The PfEMP1 family of surface proteins is central for Plasmodium falciparum virulence and must retain the ability to bind to host receptors while also diversifying to aid immune evasion. The interaction between CIDRα1 domains of PfEMP1 and endothelial protein C receptor (EPCR) is associated with severe childhood malaria. We combine crystal structures of CIDRα1:EPCR complexes with analysis of 885 CIDRα1 sequences, showing that the EPCR-binding surfaces of CIDRα1 domains are conserved in shape and bonding potential, despite dramatic sequence diversity. Additionally, these domains mimic features of the natural EPCR ligand and can block this ligand interaction.

A second complex, containing IT4var07 CIDRα1.4:EPCR complex also crystallized, and crystals diffracted to 2.9Å resolution. Despite a sequence identity of 78.5% compared to the HB3var03 CIDRα1 domain, this complex crystallized in a different space group and with different crystal packing. The structure was determined using HB3var03 CIDRα1 and EPCR as separate search models in molecular replacement. HB3var03 and IT4var07 CIDRα1 are extremely similar (rmsd = ∼0.3Å), but despite differences in space groups and crystal packing, both CIDRα1 domains bind to EPCR using the equivalent surface. The two CIDRα1 domains are built around a long three-helical core bundle. On one side of this bundle lies a four-stranded β sheet. Indeed, comparison of the structures of the CIDRα1:EPCR complexes with that of EPCR bound to the Gla domain of activated protein C (Oganesyan et al., 2002) reveals significant overlap, with both protein C and CIDRα1 domains interacting with the same region of the hydrophobic groove of EPCR.

> PDCGVICENGKCVVKENGSNCRHYNIYEPAPDVKTTEINVIVSGDEQGIITKKLQDFCMNPNNENGTNNQIWKCYYKDEKEDKCKVETKSGNSTYKEKITSFDEFFDFWVRKLLIDTIKWETELTYCINNTTNADCNNECNKNCVCFDKWVKQKEKEWKNIMDLFTNKHDIPKKYYLNINDLFNSFFFQVIYKFNEGEAKWNKLKENLKKKTESSKKNKGTKDSEAAIKVLFDHLKETATICKDNNTNEAC;> LQRLHMLQISYFRDPYHVWYQGNASLGGHLTHVLEGPDTNTTIIQLQPLQEPESWARTQSGLQSYLLQFHGLVRLVHQERTLAFPLTIRCFLGCELPPEGSRAHVFFEVAVNGSSFVSFRPERALWQADTQVTSGVVTFTLQQLNAYNRTRYELREFLEDTCVQYVQKHIS>[4x]MTPYLQFDRNQWAALRDSVPMTLSEDEIARLKGINEDLSLEEVAEIYLPLSRLLNFYISSNLRRQAVLEQFLGTNGQRIPYIISIAGSVAVGKSTTARVLQ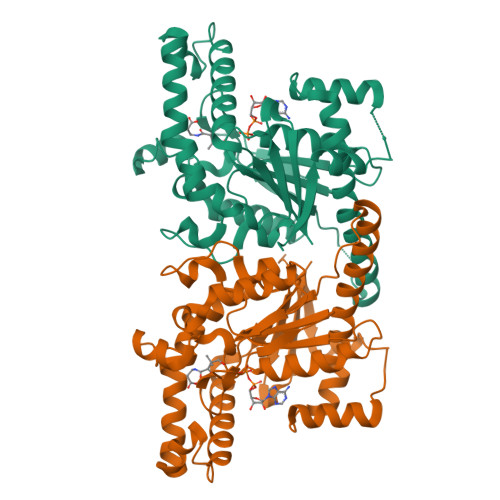ALLSRWPEHRRVELITTDGFLHPNQVLKERGLMKKKGFPESYDMHRLVKFVSDLKSGVPNVTAPVYSHLIYDVIPDGDKTVVQPDILILEGLNVLQSGMDYPHDPHHVFVSDFVDFSIYVDAPEDLLQTWYINRFLKFREGAFTDPDSYFHNYAKLTKEEAIKTAMTLWKEINWLNLKQNILPTRERASLILTKSANHAVEEVRLRK> MSGSLSRGNGGKKVLNKNQLLKRNRIRNARSIRAEAVAASSTKTGTPSDLSESGSKLNVDQFISSRQFEVKQLQLAMHNSKAASSTRIFQALPRKLRRRTASHNVRRIPKRMRNRALREMRKSDQQDVLKGSSASSRKAHGLNAKQLYKARMSIKLLRLASKSTSMKLSMPPEVTSSNCHVRQKIKTLKRMIKESSTANPNIKLLNNRMGSYDCTGVNELAPIPKGRVKYTKRQKHFAWLPTHIWNAKRSHMMKRWGYQMVWAPTQKCFKLTHRLGGDTCSSDGALCMDSSYIGTIIVKDKSNDSEGDFLKSIIGKLTAERANLRKYREGQVLFQGLIYSFNEENGEDSTKPLGPCDVFWVQKDTAIIRLHPSIYTQVFNILLQHKEKLTVQDCRYSLASVTLKGAKALESLASCLRSTEYSKSFEQFKMVSMITDHNALPQRCTFAFEAIDPRHLAAPKKLNDSQRKTVNSDDILSLHENYPQDEINAVFNELCDPESRTQSYNNQNTLKEISARRYKLLTATPNSINKTTVPFKESDDPSIPLVIIRRLKTRDWIVVLPWFWLLPLWHLLNRIPRMYHIGLRQFQQIQYENKQLYFPDDYPFTQLGYIENSFYKKEASKTKWDRKPMGKRINFEKIKDIHNTKLPAYSGEIGDFFSSDWRFLQILRNGIDYLQRNDKTLELMDSKKTGQFNAQGVRDINCVNDVLEFCKDYEAKTKAMSLSIEENIPVALCKNRKCQFRTPDSISVNSSSFSLTFFPRCIIAVSCTLLERGHPKDNARIYQVPEKDLEHWLQLAKGVYRPNGRKDHDLKIPLPEVHDLIGFITSGTYHLNCGNGMGIGFIDHHAAIRQPTRYVLIRNVGTNTYRLGEWSKISV;> MSGSLKSLDKKIAKRRQVYKPVLDNPFTNEAHMWPRVHDQPLIWQLLQSSIINKLIHIQSKENYPWELYTDFNEIVQYLSGAHGNSDPVCLFVCNKDPDVPLVLLQQIPLLCYMAPMTVKLVQLPKSAMDTFKSVSKYGMLLLRCDDRVDKKFVSQIQKNVDLLQFPWLNAIKYRPTSVKLLKTTVPIVSKKRQK;> MDRTQTFIKDCLFTKCLEDPEKPFNENRFQDTLLLLPTDGGLTSRLQRQQRKSKLNLDNLQKVSQLESADKQLEKRDYQRINKNSKIALREYINNCKKNTKKCLKLAYENKITDKEDLLHYIEEKHPTIYESLPQYVDFVPMYKELWINYIKELLNITKNLKTFNGSLALLKLSMADYNGALLRVTKSKNKTLIGLQGIVIWDSQKFFIMIVKGNIIDEIKCIPKKGTVFQFEIPISDDDDSALRYSILGDRFKYRSVDRAGRKFKSRRCDDMLYYIQN;> MVRLKSRYILFEIIFPPTDTNVEESVSKADILLSHHRASPADVSIKSILQEIRRSLSLNLGDYGSAKCNSLLQLKYFSNKTSTGIIRCHREDCDLVIMALMLMSKIGDVDGLIVNPVKVSGTIKKIEQFAMRRNSKILNIIKCSQSSHLSDNDFIINDFKKIGR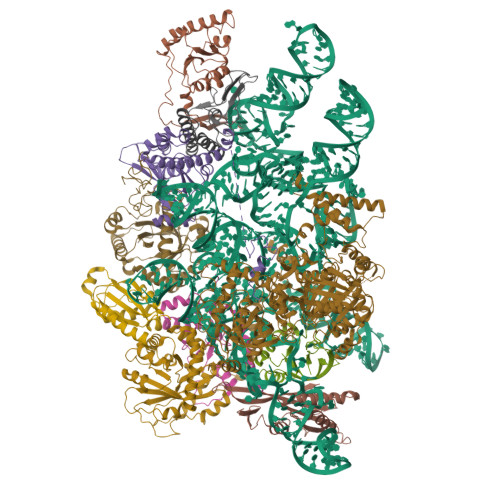ENENENEDD;> MINGVYYNEISRDLDISSSTQCLRFLKETVIPSLANNGNNSTSIQYHGISKNDNIKKSVNKLDKQINMADRSLGLQQVVCIFSYGPHIQKMLSILEIFKKGYIKNNKKIYQWNKLTSFDIKREGRNELQEERLKVPILVTLVSDSEIIDLNLHSFTKQ;> MALKKNTHNKSTKRVTKHPSLKTLTHKQIHTTIFVKSTTPYVSALKRINKFLDSVHKQGSSYVAVLGMGKAVEKTLALGCHFQDQKNKKIEVYTKTIEVLDEVITEGQADIDMESDVEDDDKETQLKKRAVSGVELRIYV;> MGKKTFREWQYFKLSITSFDQDVDDAHAIDQMTWRQWLNNALKRSYGIFGEGVEYSFLHVDDKLAYIRVNHADKDTFSSSISTYISTDELVGSPLTVSILQESSSLRLLEVTDDDRLWLKKVMEEEEQDCKCI;>[2x]MLVDLNVPWPQNSYADKVTSQAVNNLIKTLSTLHMLGYTHIAINFTVNHSEKFPNDVKLLNPIDIKRRFGELMDRTGLKLYSRITLIIDDPSKGQSLSKISQAFDIVAALPISEKGLTLSTTNLDIDLLTFQYGSRLPTFLKHKSICSCVNRGVKLEIVYGYALRDVQARRQFVSNVRSVIRSSRSRGIVIGSGAMSPLECRNILGVTSLIKNLGLPSDRCSKAMGDLASLVLLNGRLRNKSHKQTIVTGGGSGNGDDVVNDVQGIDDVQTIKVVKRSMDAEQLGHASKRHKP;> MGKKAHGGKMKPEIDENGTLLVPPPRTIANQDHFHRLNYLYQISAYQTRARQKARTDAHTPLARNYIKSMDLISKKTKTSLLPTIKRTICKKCHRLLWTPKKLEITSDGALSVMCGCGTVKRFNIGADPNYRTYSEREGNLLNS>[6x]MVNKTEKTSDLMFERFKRNVSEIVTGDGGELELTVEQRKYFLIFKNGDFLVSSCHMKHHLV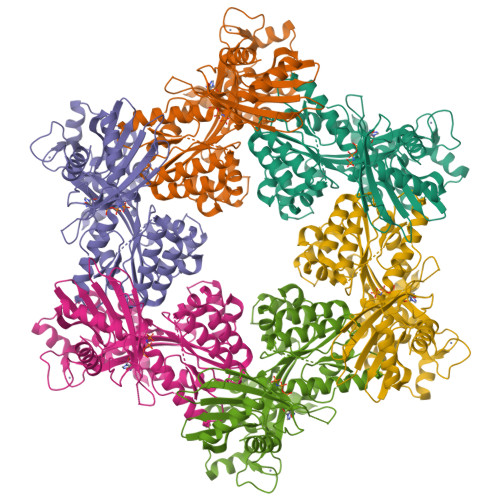QMLREIATRKGYPNLTIYEVNLKDIRLLYEASLKTVQNNGQDLLPVEKRASMLLFECAEMRVSDLHIKVYDAEADIYIRKDGDMELLRQIESNTAHSILASLYNNADDSDATYKINAYQAARIVASKSRLALPPVIQAVRLQFNPLGQGGRYLIARFLYTDKSEKQKEMDPTRFGFHHSHAESFSRMRNLPIGINIISGPTGSGKSTTLKNLLELLYIEKKKKVNIISIEDPPEYEIDGTAQLPITNVETEAQRGEEYRKAITAALRSDPDIIMPGEARDAEVINLLFTAAMTGHQVWTSLHANNALAIFDRLKDQGVDEFKLTDPELITGLVAQRLVRKLCAQCSITLTEYIASGGGISDTDRKIISGHETSVRFPNPRAKKCCRDGYNGRTILAEVIEPDSKLLRLVAEGKREDAQHYWLTSLHGMALKEHAWLKIISGEICVMDAVNKISGIDNITEERKKYLFSRDNEI>AVPRGSHMMIRYVDLDAAEGAALDELTRSVLRDHGASSSPSLLDDLSLVAHRMPPRLIRELRRFRTAEEASCLVVRGLPVDDRRLGPTPLDWREPPREPESEVHEVFLTLATAHLGDIFGWSTLQNGRLVHDVLPVPSHENDQSGHGTVELAWHTEDGFHPYRCDYLLLLGLRNHDAVPTGVAGVDQVVLSDEHREVLSQPRFLIRPDTEHLRHARTLAADRGSPHAVQLMQDEPEPCAVLFGHPDRPYLRIDPAFMSPLPGDPEAAAALEALTAELQRNLTDVVLSPGDLLVIDNYRVVHGRAAFKARFDGTDRWLKKAVV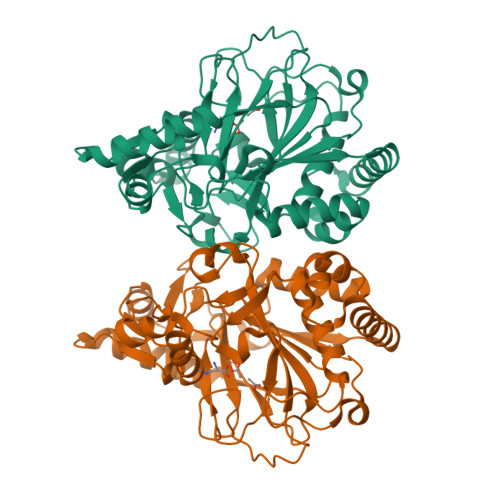TRDLRKSRAHRKSAAERVLL[2x]>[4x]MSL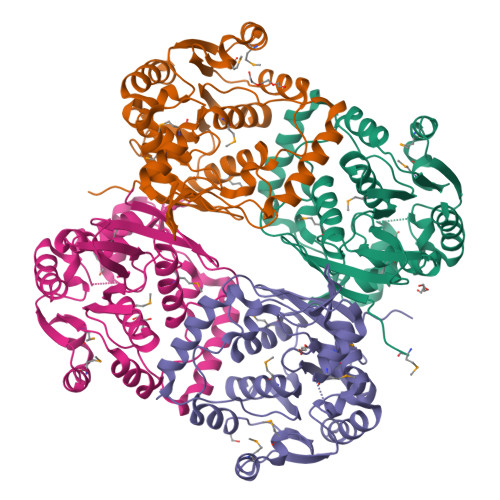QVEEVRISLPHIELAAHLFGPPDGKPVIALHGWLDNAMSFSRLAPKLAGLRIVALDFAGHGHSAHRAEGASYLLWDYALDVLMVAEQLGWERFSLLGHSMGAIVSVLLAGALPERIERLALIDGLIPYTGEADKAPQKLGEALKAQLALRHKRKPVYAELEKAVEARMRGVGEISREAAELLAQRGLEPVPGGYTWRTDARLTLPSPLRLTQAHALNFVRSVECPVSLVLAEQGMLAVEPRMRALLETLPFERHHLPGGHHLHLDDEAGAQAVARVFAAFFAR1-[(2-chlorophenyl)methyl]-N-hydroxy-4-phenyl-1H-pyrrole-3-carboxamide | 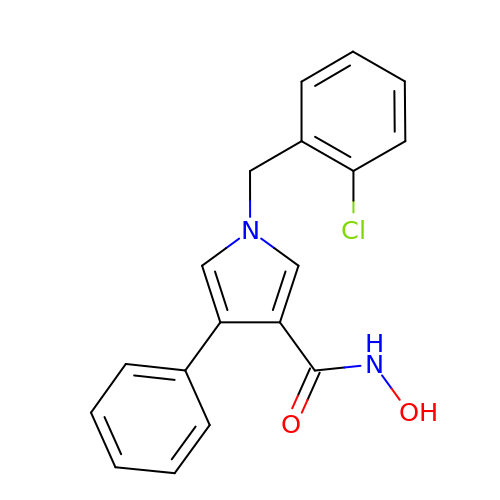C18 H15 Cl N2 O2 | SFMZKKRSVVMNSR-UHFFFAOYSA-N> GAMSETSVNRGPEKIRPECFELLRVLGKGGYGKVFQV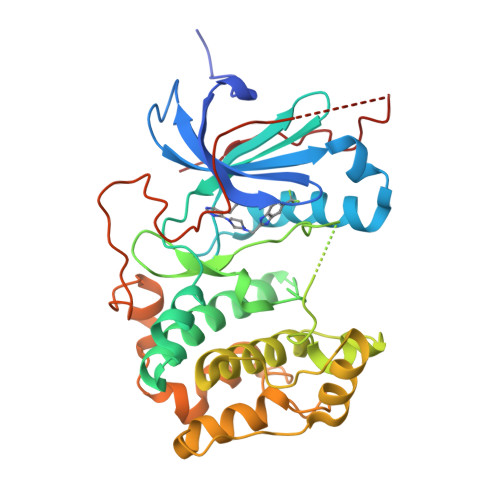RKVTGANTGKIFAMKVLKKAMIVRNAKDTAHTKAERNILEEVKHPFIVDLIYAFQTGGKLYLILEYLSGGELFMQLEREGIFMEDTACFYLAEISMALGHLHQKGIIYRDLKPENIMLNHQGHVKLTDFGLCKESIHDGTVTHTFCGTIEYMAPEILMRSGHNRAVDWWSLGALMYDMLTGAPPFTGENRKKTIDKILKCKLNLPPYLTQEARDLLKKLLKRNAASRLGAGPGDAGEVQAHPFFRHINWEELLARKVEPPFKPLLQSEEDVSQFDSKFTRQTPVDSPDDSTLSESANQVFLGFAYVAPS β-Propeller proteins are common natural disc-like pseudo-symmetric proteins that contain multiple repeats (‘blades’) each consisting of a 4-stranded anti-parallel β-sheet. In the larger propellers a so-called “Velcro closure” is found, in which the N- and C-terminal β-strands are part of the same β-sheet, keeping the propeller closed. This “Velcro” can occur in different positions; in the “Velcro 1-3” variant, the closing β-sheet consists of one N-terminal and three C-terminal strands, while for the “Velcro 3-1” variant, the opposite is true. Starting from a highly repetitive β-propeller sequence, we designed a consensus motif sequence that formed a perfectly symmetric 7-bladed β-propeller.

While the space group and packing differ between the crystals, the structure is identical for each protein. The crystal structures also show that the proteins are highly internally symmetric with a backbone RMSD between individual repeats below 0.3 Å. The characteristic hydrogen bridge network in WD40 repeats, between a conserved histidine, serine, aspartate and tryptophan is clearly visible in the electron density, see Fig. 4. Analysing the thermal and chemical stability of the WRAP-T permutants revealed that nvWRAP-T, lacking the velcro closure, is just as stable as the variant v13WRAP-T. While v31WRAP-T is considerably more resistant to GdnHCl induced denaturation compared to the other proteins, its increased thermal stability is not that significant. From this, the fraction of denatured protein could be calculated by assuming the protein is completely unfolded at the highest concentration. When possible this data was fitted with a Boltzmann-sigmoid curve to determine the concentration at which 50% of the protein is denatured and the proportionality constant (m), see Table 2. v13WRAP-T remained stable at high GdnHCl concentration thus fitting the data was not possible. A striking difference however is the stability of the “non-Velcro” variant, the least stable for Pizza but as stable as the natural “Velcro” position in WRAP-T. This may be due to differences between the sequences, as the two different “non-Velcro” variants of Pizza have different stabilities as well.

>MGQLLQTLTGHSSSVTGVAFSPDGQTIASASDDKTVKLWNRNGQLLQTLTGHSSSVTGVAFSPDGQTIASASDDKTVKLWNRNGQLLQTLTGHSSSVTGVAFSPDGQTIASASDDKTVKLWNRNGQLLQTLTGHSSSVTGVAFSPDGQTIASASDDKTVKLWNRNGQLLQTLTGHSSSVTGVAFSPDGQTIASASDDKTVKLWNRNGQLLQTLTGHSSSVTGVAFSPDGQTIASASDDKTVKLWNRNGQLLQTLTGHSSSVTGVAFSPDGQTIASASDDKTVKLWNRN[2x]> MKIIVCITGASGVIYAKRLLEVLKDRAEVNL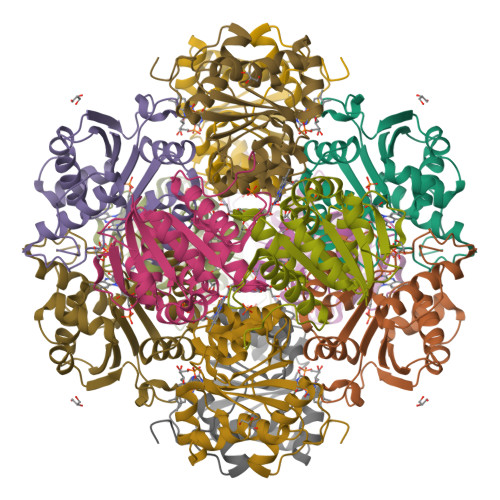IISNSAKKIIKEELDIDWKEIKKLATDYYENDDFFSPLASGSNKFDAVVVVPCSMKTLSAIANGYSANLIVRVCDIALKERRKLIIMPREMPFNSIHLENMLKLSNLGAIVMPPIPAFYNKPKNVNDIINFVVGRVLDILGIDNSLFKRWGTV> QDNSRYTHFLTQHYDAKPQGRDDRYCESIMRRRGLTSPCKDINTFV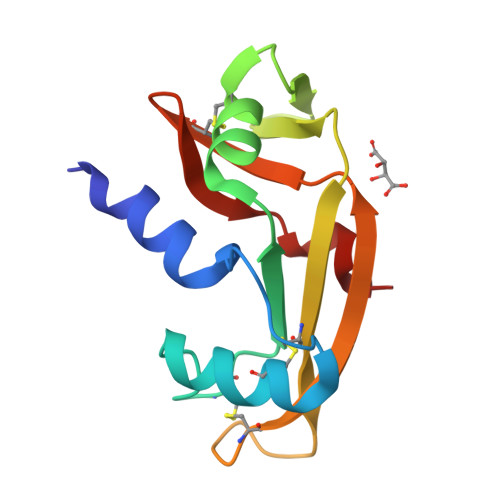HGNKRSIKAICENKNGNPHRQNLRISKSSFQVTTCKLHGGSPWPPCQYRATAGFRNVVVACENGLPVHLDQSIFRRP> MSTRKAVIGYYFIPTNQINNYTETDTSVVPFPVSNITP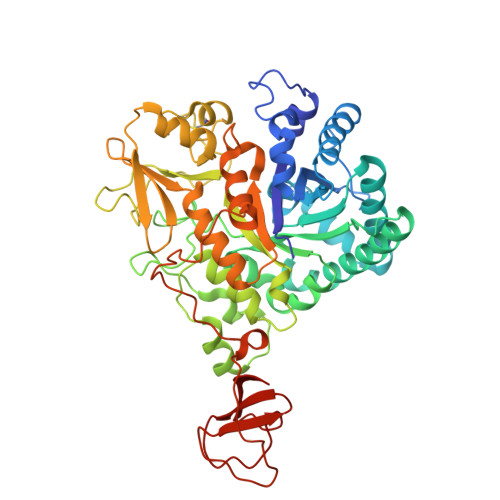AKAKQLTHINFSFLDINSNLECAWDPATNDAKARDVVNRLTALKAHNPSLRIMFSIGGWYYSNDLGVSHANYVNAVKTPASRTKFAQSCVRIMKDYGFDGVDIDWEYPQAAEVDGFIAALQEIRTLLNQQTITDGRQALPYQLTIAGAGGAFFLSRYYSKLAQIVAPLDYINLMTYDLAGPWEKVTNHQAALFGDAAGPTFYNALREANLGWSWEELTRAFPSPFSLTVDAAVQQHLMMEGVPSAKIVMGVPFYGRAFKGVSGGNGGQYSSHSTPGEDPYPSTDYWLVGCEECVRDKDPRIASYRQLEQMLQGNYGYQRLWNDKTKTPYLYHAQNGLFVTYDDAESFKYKAKYIKQQQLGGVMFWHLGQDNRNGDLLAALDRYFNAADYDDSQLDMGTGLRYTGVGPGNLPIMTAPAYVPGTTYAQGALVSYQGYVWQTKWGYITSAPGSDSAWLKVGRVA> GSMASLPVLQKESVFQSGAHAYRIPALLYLPGQQSLLAFAEQRASKKDEHAELIVLRRGDYDAPTHQVQWQAQEVVAQARLDGHRSMNPCPLYDAQTGTLFLFFIAIPGQVTQEQQLQTRANVTRLCQVTSTDHGRTWSSP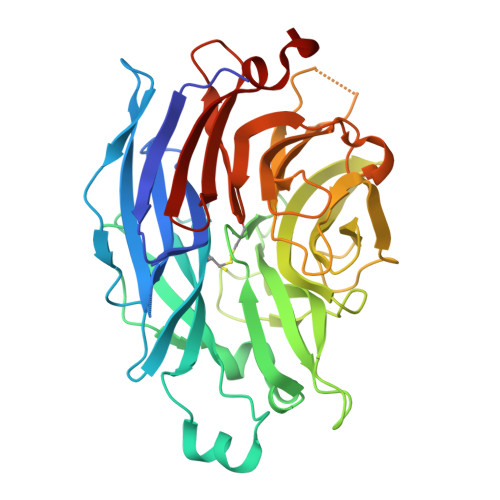RDLTDAAIGPAYREWSTFAVGPGHCLQLNDRARSLVVPAYAYRKLHPIQRPIPSAFCFLSHDHGRTWARGHFVAQDTLECQVAEVETGEQRVVTLNARSHLRARVQAQSTNDGLDFQESQLVKKLVEPPPQGCQGSVISFPSPRSGPGSPAQWLLYTHPTHSWQRADLGAYLNPRPPAPEAWSEPVLLAKGSCAYSDLQSMGTGPDGSPLFGCLYEANDYEEIVFLMFTLKQAFPAEYLPQ>GSHMLDMTRIILPGKTIGIIGGGQLGRMMALAAKEMGYKIAVLDPTKNSPCAQVADIEIVASYDDLKAIQHLAEISDVVTYEFENIDYRCLQWLEKHAYLPQGSQLLSKTQNRFTEKNAIEKAGLPVATYRLVQNQEQLTEAIAELSYPSVLKTTTGGYDGKGQVVLRSEADVDEARKLANAAECILEKWVPFEKEVSVIVIRSVSGETKVFPVAENIHVNNILHESIVPARITEELSQKAIAYAKVLADELELVGTLAVEMFATADGEIYINELAPRPHNSGHYTQDACETSQFGQHIRAICNLPLGETNLLKPVVMVNILGEHIEGVLRQVNRLTGCYLHLYGKEEAKAQRKMGHVNILNDNIEVALEKAKSLHIWDHQEQLLEGKR[2x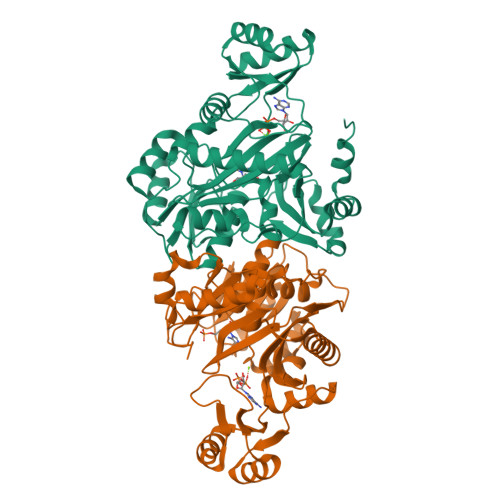]>MTSAEIRAAFLEFFRQRGHAVRPSSSLVPGNDPTLLFTNAGMVQFKDVFLGREKVDFNRAATSQRCVRAGGKHNDLENVGYTARHHTFFEMLGNFSFGDYFKRDAINFAWDFLTKEMGIPPAKLWVTVFDEDSEAEAIWLEEVKIDPTRFSRIGAKDNFWAMGDVGPCGPCTEIFYDHGEHVAGGPPGSPDEDGDRYIEIWNLVFMQYERDKDGNLTPMPAPSVDTGMGLERIAAVMQGVHSNYEIDIFQNLVKTAAALAGTTDLSNSSLRVIADHIRSCAFLVADGVLPSNEGRGYVLRRIVRRAIRHGYRLGIQDTFFYKLVAPLAAEMGAAYPELVKAQEQVERVLKKEEERFAETLGQGMKILENCVAKLDGHVIPGDVVFLLYDTYGFPVDLTADFAREHNLSVDHAGFEVEMSAQRDRARAGGHHHHHH[2x]

Aminoacyl-tRNA synthetases (AARSs) play a crucial role in the translation of genetic information by attaching specific amino acids to their corresponding transfer RNA (tRNA) molecules. Alanyl-tRNA synthetase (AlaRS) often misactivates Gly or Ser instead of its cognate amino acid, Ala. To get structural explanation why the L219M mutation prevents AlaRS from misactivating Ser to produce seryl-adenylate, we determined the crystal structures of both the wild-type and L219M mutant AlaRS proteins in complex with ATP and Ala. AlaRS429 and AlaRS429L219M consist of the N-terminal nine-stranded β-sheet structure harboring the catalytic site (residues 1–241) and the C-terminal α-helix bundle (residues 242–429) responsible for tRNA recognition.

Here we show a groundbreaking discovery where a single-point mutation, L219M, in AlaRS from Methylomonas sp. DH-1, effectively eliminates Ser misactivation. Hereafter, the structure of AlaRS429L219M was employed to describe the binding modes of ATP and Ala since electron density for Ala was clearer in this structure. The presence of ATP and Ala in their intact forms indicates that this structure depicts the conformational state before activation. When the structure of AlaRS429L219M is superposed onto those of E. coli AlaRS, it was obvious that AlaRS429L219M resembles the open structure of the apo state rather than the closed structure depicting the conformational state after aminoacylation. First, the adenine base is stacked between Phe89 in motif 2 and Arg232 in motif 3, which anchors ATP in the active site. The α-NH3+ group of Ala interacts with the α-phosphate group of ATP and its methyl side chain forms hydrophobic contact with Val204. The distance between the methyl side chain of Ala and Val204 is 3.4 Å, which suggests that if Ser were positioned in the same space, the extra hydroxyl group of Ser would clash with Val204. Interestingly, the B-values of Cα atoms of Val204 in AlaRS429 and AlaRS429L219M are 19.96 and 26.68 Å2, respectively, suggesting that Val204 is more flexible in AlaRS429L219M than in AlaRS429. That is, the more dynamic Val204 of AlaRS429L219M invades the space intended for the extra hydroxyl group of Ser, whereas the relatively static Val204 in AlaRS429 allows the binding of Ser without inducing clash with the hydroxyl group. Structural analyses of the pre-reaction state revealed that the L219M mutation increases the flexibility of Val204. This enhanced flexibility enables Val204 to function as a “molecular discriminator,” selectively blocking the binding of Ser to the active site of AlaRS429L219M while still permitting the accommodation of Ala.>[3x]GAMVVKDQVDLRKRKHLEENERRHEDAIKRRKEAVNMNVEKPTVYHCKVFQFKNLQNPKIRFKLKMNSKELSLKGLCLRIRDDGPGIIIVVGNEKS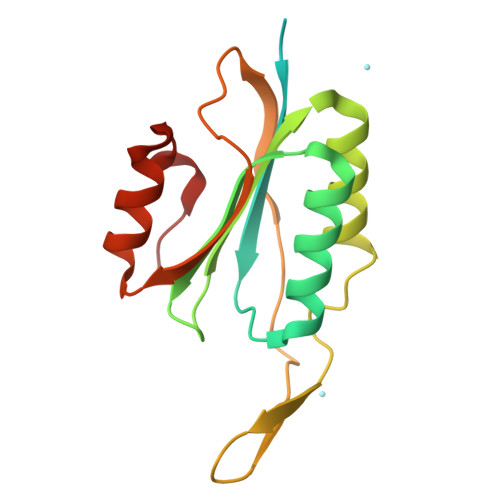CKFYENLVMKRIKWNEDFELHTNTGDIKMDMHNNSISKTWEGYLQDCKFKGWFMKVCNDQDSLLRTLGQFDSEHFYSPVQT>[2x]MRSRRVDVMDVMNRLILAMDLMNRDDALRVTGEVREYIDTVKIGYPLVLSEGMDIIAEFRKRFGCRIIADFKVADIPETNEKICRATFKAG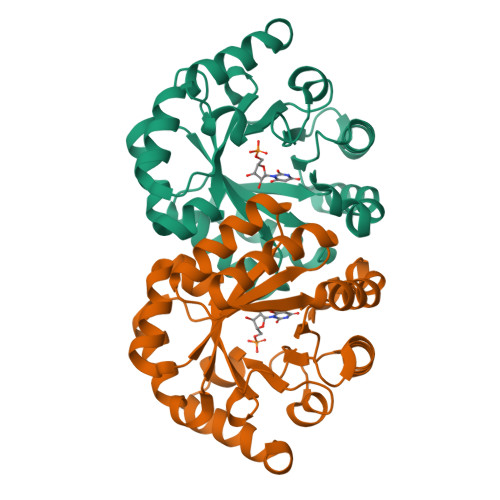ADAIIVHGFPGADSVRACLNVAEEMGREVFLLTEMSSPGAEMFIQGAADEIARMGVDLGVKNYVGPSTRPERLSRLREIIGQDSFLISPGVGAQGGDPGETLRFADAIIVGRSIYLADNPAAAAAGIIESIKDLLNP>MGDTKEQRILRYVQQNAKPGDPQSVLEAIDTYCTQKEWAMNVGDAKGQIMDAVIREYSPSLVLELGAYCGYSAVRMARLLQPGARLLTMEMNPDYAAITQQMLNFAGLQDKVTILNGASQDLIPQLKKKYDVDTLDMVFLDHWKDRYLPDTLLLEKCGLLRKGTVLLADNVIVPGTPDFLAYVRGSSSFECTHYSSYLEYMKVVD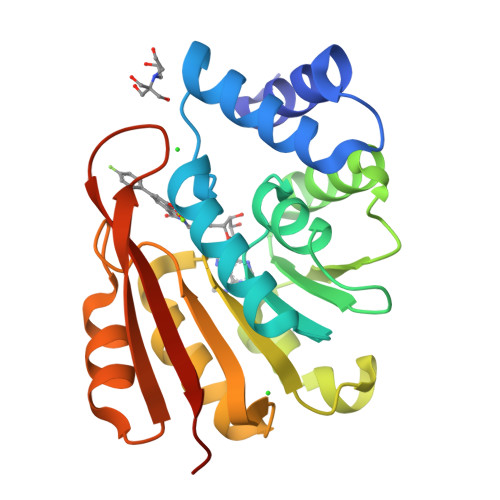GLEKAIYQGPSSPDKS[2x]> MDVLEMFDVNYESPILESFDSTTQSLNDVHVFMSRIQMSAYDADGEGRIEYRNLKLYEISSGIFISTDRLDTGASGVEDDHEMVDYYSSARLTREFLGESLDSQKSDYFEGIKKVFSFYKNKCNESRYIKEFFEEIQFRNICGFPKQAGTSSTDIFDQFNSVDVLLQDPVTSVWNKKVGSKKANIVIIPPATNLPITEACATAGFQPEGFPKLGSGSFFTVQFDPFFSTRFKAHETDDVALLDPTLTLLHEMTHGLHFQKGIANPVNRSGETPAWATTWGRVTGDNDAFKETPMEELLTFNKHTIDDDIEISDHLKSTYIGFLYNGRNEDDPTESVDGVYQNVSSFLNQYRGFEISSDFQHFIESCYGVKYNQESKKFIVNPRNIKRYVQDGFFIDEAKFARILNIKTRSYYTLMPDNLGVWSYRVDILNRLRETFDEDRGLLSQELDFHTALTPVVSENPALELEVAGMQRMVSLPKIKASYLPSDIKIKNFTGQKISHDTILDTNISGIIISKIKYKSDFVVDESMPRSSLNTTNYNLSPIKGTKFETDIRDKTSVKVTVSEITAPMINHVMKLDNSKVLTERPSLNEDLEETFKNTKDVYIPKTTAMMKLKEGADQTLGAVGFAVWSGQILEDLYNLAQKKEVSIDQIKDDLMSILPFYCAYKNLSAEKYEQAFANATLDAFLIFATDGGGFAGLGITVGAIAINSMYAKAETMEAYDSMFGKYVDQYQNDIKNFTLNAYVQWENNILSRLWNESRLAITGFRNMLKTVKTVMEFDATNQAYSEEDRKIIKAKCEEIFSEFPMLMQTFAKNSMTANLENASKIFNDIVWQKIKEELDQYVIDSKKYFLDSLEEAYNNGSISAESYYKYQTEAREKFVSPREVIDLYIAAHDTVVKRKRYIRRYSRKYDLATDFKGNTVHLNGLGEGTQDIQDLYGNYSVYADKKTVSTQEGHFDQTIKIAKDTNTINKVVLAVSSNNG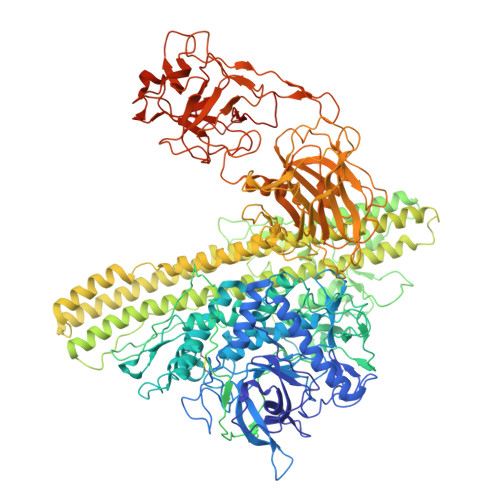KEYALNKDEQYTISFWLRMPVPSSSEERRIFSYSAVSGVNKEVEELILQVKNNEFVLATANLLRNSEFVIEPRIALNRWVKITIVNENTRIKVYQNDNLLGLIKDSSRKKPIAQRGTFKFYNYNVDYQLDDISYYNGTISQRDIKYTFKEDHGQFVYDHWGERLQYNKAYYLLSDDNKSAFETVYETKRLKLKSVPGVDIKYLGMNDRVYGYYGGLQFKLVPLDSKNMNNYVRWGDKFTMQSIETTNLSLAIIQDNAYFAPTQLKLISNEGKSEEEIFTFDRNIKLQNAAILVGTGNSKQGPISAYKRGYSGDLWINGARLDGYVTVVNKSNYSNDEIQEKFKWIFVPKDANWVEGSYPYDVPDYALESGKETAAAKFERQHMDSSTSAA> GPGSDADKERLARENHSEIERRRRNKMTAYITELSDMVPTCSALARKPDKLTILRMAVSHMKSLRGTGNTSTDGSYKPSFLTDQELKHLILEAADGFLFIVSCETGRVVYVSDSVTPVLNQPQSEWFGSTLY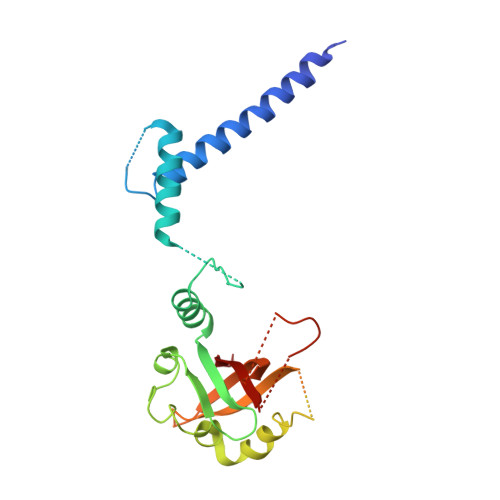DQVHPDDVDKLREQLSTSENALTGRVLDLKTGTVKKEGQQSSMRMSMGSRRSFICRMRCGTSSHFVVVHCTGYIKAWPPAGVSLPDDDPEAGQGSKFCLVAIGRLQV>AEEFPVPNGFESAYREVDGVKLHYVKGGQGPLVMLVHGFGQTWYEWHQLMPELAKRFTVIAPDLPGLGQSEPPKTGYSGEQVAVYLHKLARQFSPDRPFDLVAHSIGIWNTYPMVVKNQ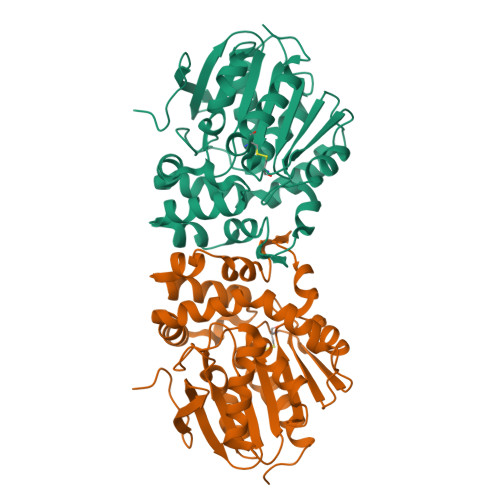ADIARLVYMEAPIPDARIYRFPAFTAQGESLVWHFSFFAADDRLAETLIAGKERFFLEHFIKSHASNTEVFSERLLDLYARSYAKPHSLNASFEYYRALNESVRQNAELAKTRLQMPTMTLAGGGHGGMGTFQLEQMKAYAEDVEGHVLPGCGHWLPEECAAPMNRLVIDFLSRGRHHHHHH[4x]> GPESCTSRPHITVVEGEPFYLKHCSCSLAHEIETTTKSWYKSSGSQEHVELNPRSSSRIALHDCVLEFWPVELNDTGSYFFQMKN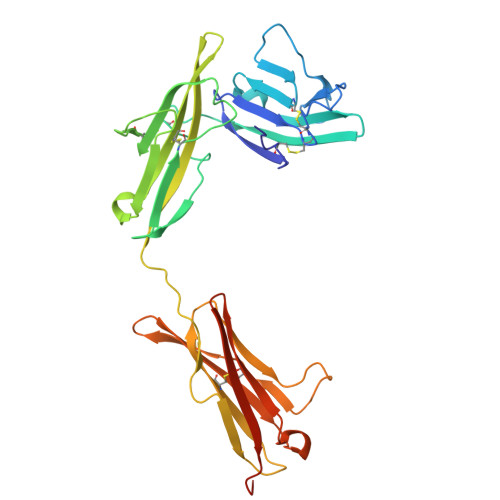YTQKWKLNVIRRNKHSCFTERQVTSKIVEVKKFFQITCENSYYQTLVNSTSLYKNCKKLLLENNKNPTIKKNAEFEDQGYYSCVHFLHHNGKLFNITKTFNITIVEDRSNIVPVLLGPKLNHVAVELGKNVRLNCSALLNEEDVIYWMFGEENGSDPNIHEEKEMRIMTPEGKWHASKVLRIENIGESNLNVLYNCTVASTGGTDTKSFILVRKADMADIPGHVFTR>[2x]SKWRSQLDRFVKENQQDLAALF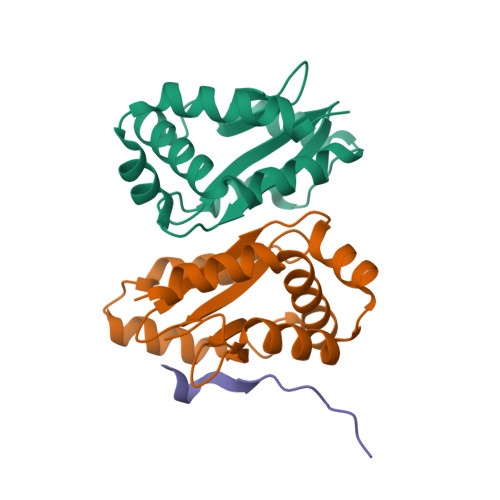WGLWLENGDSQGTIGIDLQPTPHFVYCPKDAVEKLNNNVENRLQELLGIIEHNQPEIEVLMIGIGKGEIKLIQFAPEPPPPVCFEQVGKDIDGLLELLEQRMSGEIVV;> FRENVNAIRPFGRRP A trait of BP bacteria is a conserved gene cluster coding for the biosynthesis of polyketides (malleicyprols) with a reactive cyclopropanol unit that is critical for virulence. We show that BurG, an unusual NAD+-dependent member of the ketol-acid reductoisomerase family, constructs the strained cyclopropanol ring. A sequence similarity search using BLAST predicted that BurG belongs to the family of ketol-acid reductoisomerases (KARIs; EC 1.1.1.86), well-characterized enzymes that play key roles in the biosynthesis of branched-chain amino acids. Biochemical assays and a suite of eight crystal structures of native and mutated BurG with bound analogues and inhibitors provide snapshots of each step of the complex reaction mechanism, involving a concealed oxidoreduction and a C–S bond cleavage.

To investigate the redox proficiency of BurG and its ability to regenerate NAD+ from NADH we devised an absorbance-based assay with the substrate surrogate hydroxypyruvate 8. BurG was incubated with 8 and NADH and the light absorption of the dinucleotide at 340 nm was monitored spectrophotometrically. A clearly observed signal decrease corresponds to the formation of NAD+ and glyceric acid 9, the reduced form of 8. The transformation of rac-12 into the trapped enolate 13 provides evidence for an intermediary oxidation during the catalytic cycle of BurG. We obtained similar results in co-crystallization assays with BurG, NAD+ and the substrate surrogate hydroxypyruvate 8. Subsequent hydride transfer from the C-α of gonydiol to NAD+ (yielding NADH), and deprotonation at the β carbon by E232 would result in an enolate intermediate (14), as mimicked by hydroxypyruvate and the oxidized carba-gonydiol analogue 13.

> GSHMASNDLIYQDEHASLQPLEGRTVAVIGYGIQGRAFAANLRDSGVAVRVGNIDDRYFELARAEGHRVTNIAEAVAHADIVLLLIPDEAHGAVFDVDIAPNLRDGALLCVAHGHSLVQGDVRPLPGRDLAMLAPRMYGDPIRRYYLAGQGAPAYFDIVADHTGRARDRVLAIARAVGFTRAGVMALGYRQETFLDLFQEQFLAPALVDLVETGFQVLVERGFNPKAALLEVYGSGEMGKMMLDGADIGLDEVVALQGSPTCQVGYHRWRGRTLPTAVRELAARVLDQIEGGDFSAYLKEQASNDYASLDDARRAALKRPLNVAHAQVRAAFRFPTEAAGGLYQAAQAPADVEPEAAR N-benzyl-2-({N-[2-(1H-indol-3-yl)ethyl]glycyl}amino)-4,5,6,7-tetrahydro-1-benzothiophene-3-carboxamide | C28 H30 N4 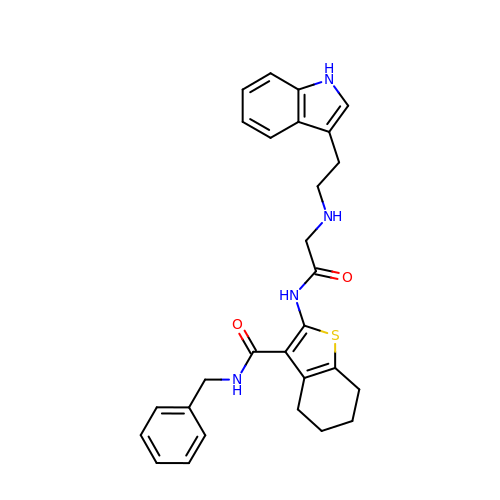O2 S | XGJXJNNCXIECFE-UHFFFAOYSA-N> MEAAHSKSTEECLAYFGVSETTGLTPDQVKRHLEKYGHNELPAEEGKSLWELVIEQFEDLLVRILLLAACISFVLAWFEEGEETITAFVEPFVILLILIANAIVGVWQERNAENAIEALKEYEPEMGKVYRADRKSVQRIKARDIVPGDIVEVAVGDKVPADIRILSIKSTTLRVDQSILTGESVSVIKHTEPVPDPRAVNQDKKNMLFSGTNIAAGKALGIVATTGVSTEIGKIRDQMAATEQDKTPLQQKLDEFGEQLSKVISLICVAVWLINIGHFNDPVHGGSWIRGAIYYFKIAVALAVAAIPEGLPAVITTCLALGTRRMAKKNAIVRSLPSVETLGCTSVICSDKTGTLTTNQMSVCKMFIIDKVDGD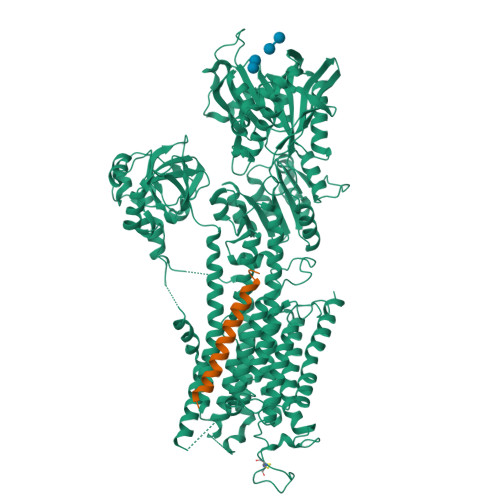FCSLNEFSITGSTYAPEGEVLKNDKPIRSGQFDGLVELATICALCNDSSLDFNETKGVYEKVGEATETALTTLVEKMNVFNTEVRNLSKVERANACNSVIRQLMKKEFTLEFSRDRKSMSVYCSPAKSSRAAVGNKMFVKGAPEGVIDRCNYVRVGTTRVPMTGPVKEKILSVIKEWGTGRDTLRCLALATRDTPPKREEMVLDDSSRFMEYETDLTFVGVVGMLDPPRKEVMGSIQLCRDAGIRVIMITGDNKGTAIAICRRIGIFGENEEVADRAYTGREFDDLPLAEQREACRRACCFARVEPSHKSKIVEYLQSYDEITAMTGDGVNDAPALKKAEIGIAMGSGTAVAKTASEMVLADDNFSTIVAAVEEGRAIYNNMKQFIRYLISSNVGEVVCIFLTAALGLPEALIPVQLLWVNLVTDGLPATALGFNPPDLDIMDRPPRSPKEPLISGWLFFRYMAIGGYVGAATVGAAAWWFMYAEDGPGVTYHQLTHFMQCTEDHPHFEGLDCEIFEAPEPMTMALSVLVTIEMCNALNSLSENQSLMRMPPWVNIWLLGSICLSMSLHFLILYVDPLPMIFKLKALDLTQWLMVLKISLPVIGLDEILKFIARNYLEG;>MDKVQYLTRSAIRRASTIEMPQQARQALQCLFINFCAILICLLLICIIGMLL[2x]>MRRRSRMLLCFAFLWVLGIAYYMYSGGGSALAGGAGGGAGRKEDWNEIDPIKKKDLHHSNGEEKAQSMETLPPGKVRWPDFNQEAYVGGTMVRSGQDPYARNKFNQVESDKLRMDRAIPDTRHDQCQRKQWRVDLPATSVVITFHNEARSALLRTVVSVLKKSPPHLIKEIILVDDYSNDPEDGALLGKIEKVRVLRNDRREGLMRSRVRGADAAQAKVLTFLDSHCECNEHWLEPLLERVAEDRTRVVSPIADVINMDNFQYVGASADLKGGFDWNLVFKWDYMTPEQRRSRQGNPVAPIKTPMIAGGAFVMDKFYFEELGKYDMMMDVWGGENLEISFRVWQCGGSLEIIPCSRVGHVFRKQHPYTFPGGSGTVFARNTRRAAEVWMDEYKNFYYAAVPSARNVPYG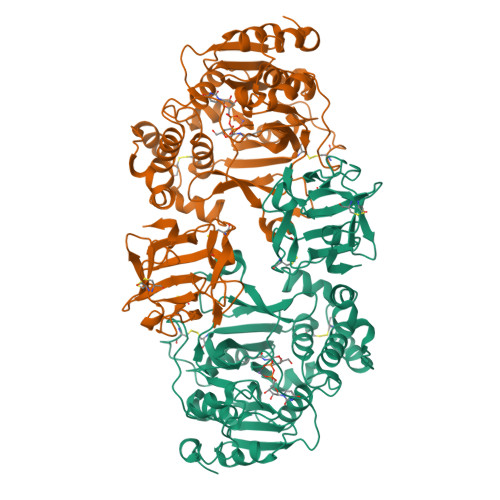NIQSRLELRKKLSCKPFKWYLENVYPELRVPDHQDIAFGALQQGTNCLDTLGHFADGVVGVYECHNAGGNQEWALTKEKSVKHMDLCLTVVDRAPGSLIKLQGCRENDSRQKWEQIEGNSKLRHVGSNLCLDSRTAKSGGLSVEVCGPALSQQWKFTLNLQQ[6x]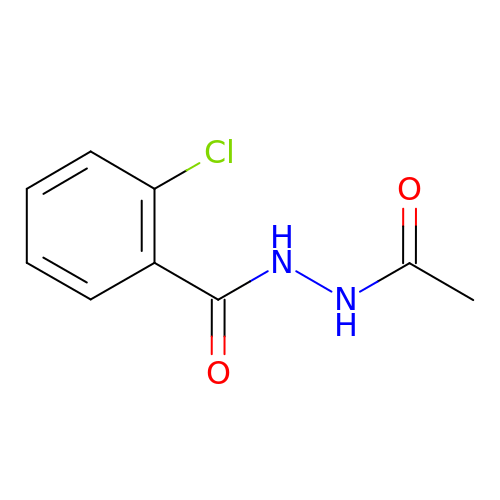N'-acetyl-2-chlorobenzohydrazide | C9 H9 Cl N2 O2 | JARLZRSFUFGXQH-UHFFFAOYSA-N> MGHHHHHHMESVTVYAAASLTNAINDLEKIYEKQNKVEVKTSYAGSSTLAKQIEAGAPADIFISADTQWMDYLQNKKLVAAN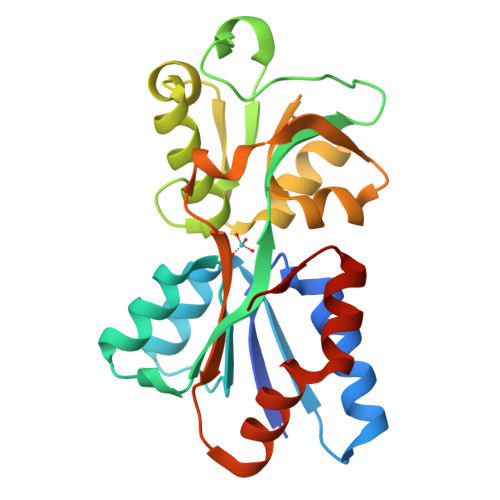DRINLLGNRLVLITPKGQSLNIKLDKATDPNKVFTGKICTGDTKSVPVGKYAKQAFTNLGWWNRIEPKLVETEDVRVALNFVARGECQVGIVYATDAAISKDVKVAGIFPENTHSPIIYPLGLIKKNSNSAKFYQFLQSNQAKAVFKKYGFSMLAPVKP> FNIVGTTYP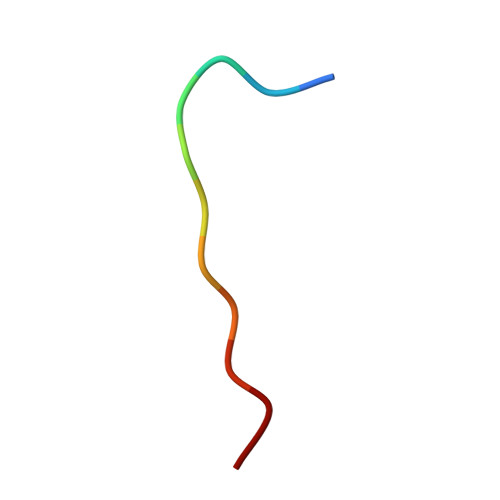IN> SQIPASEQETLVRPKPLLLKLLKSVGAQKDTYTMKEVLFYLGQYIMTKRLYDEKQQHIVYCSNDLLGDLFGVPSFSVKEHRKIYTMIYRNLVVVNQQESSDSG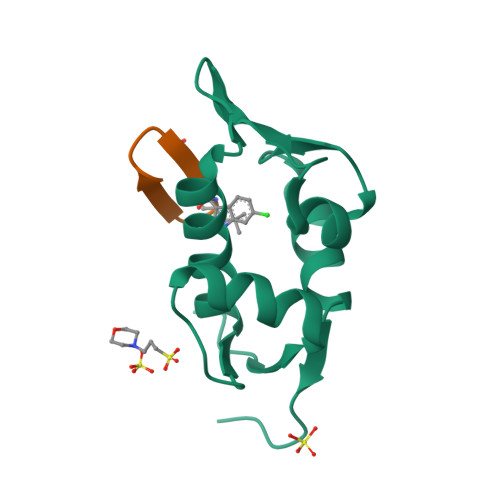TSVSENHHHHHH;> PFEWLDWEFP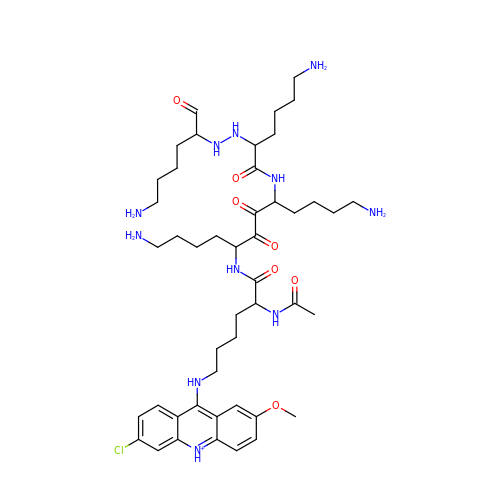9-[(5-(ACETYLAMINO)-6-{[(1S,4R)-8-AMINO-4-[((2R)-6-AMINO-2-{2-[(1S)-5-AMINO-1-FORMYLPENTYL]HYDRAZINO}HEXANOYL)AMINO]-1-(4-AMINOBUTYL)-2,3-DIOXOOCTYL]AMINO}-6-OXOHEXYL)AMINO]-6-CHLORO-2-METHOXYACRIDINIUM | C46 H73 Cl N11 O7 | UBQMMWHASWFFFO-QDCRQMTFSA-O> DQQLVDQLSQLKLNVKMLDNRAGENGVDCAALGADWASCNRVLFTLSNDGQAIDGKDWVIYFHSPRQTLRVDNDQFKIAHLTGDLYKLEPTAKFSGFPAGKAVEIPVVAEYWQLFRNDFLPRWYATSGDAKPKMLANTDTENLDQFVAPFTGDQWKRTKDDKNILMTPASRFVSNADLQTLPAGALRGKIVPTPMQVKVHAQDADLRKGVALDLSTLVKPAADVVSQRFALLGVPVQTNGYPIKTDIQPGKFKGAMAVSGAYELKIGKKEAQVIGFDQAGVFYGLQSILSLVPSDGSGKIATLDASDAPRFPYRGIFLDVARNFHKKDAVLRLLDQMAAYKLNKFHFHLSDDEGWRIEIPGLPELTEVGGQRCHDLSETTCLLPQYGQGPDVYGGFFSRQDYIDIIKYAQARQIEVIPEIDMPAHARAAVVSMEARYKKLHAAGKEQEANEFRLVDPTDTSNTTSVQFFNRQSYLNPCLDSSQRFVDKVIGEIAQMH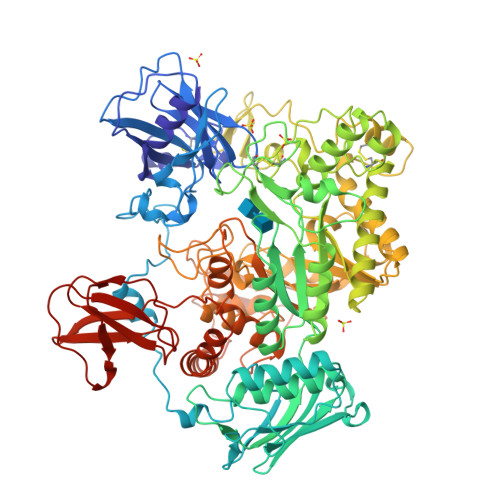KEAGQPIKTWHFGGDEAKNIRLGAGYTDKAKPEPGKGIIDQGNEDKPWAKSQVCQTMIKEGKVADMEHLPSYFGQEVSKLVKAHGIDRMQAWQDGLKDAESSKAFATSRVGVNFWDTLYWGGFDSVNDWANKGYEVVVSNPDYVYMDFPYEVNPDERGYYWGTRFSDERKVFSFAPDNMPQNAETSVDRDGNHFNAKSDKPWPGAYGLSAQLWSETQRTDPQMEYMIFPRALSVAERSWHRAGWEQDYRAGREYKGGETHFVDTQALEKDWLRFANILGQRELAKLDKGGVAYRLPVPGARVAGGKLEANIALPGLGIEYSTDGGKQWQRYDAKAKPAVSGEVQVRSVSPDGKRYSRAEKV> MSNITIYHNPACGTSRNTLEMIRNSGTEPTI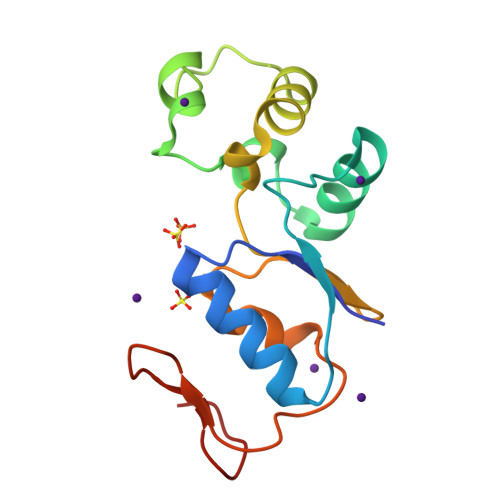ILYLENPPSRDELVKLIADMGISVRALLKKNVEPYEQLGLAEDKFTDDQLIDFMLQHPILINRPIVVTPLGTRLCRPSEVVLDILQDAQKGAFTKEDGEKVVDEAGKRLK> GSEPTFVVNASLLPSKVLGLQVQRPQSFNYQPGDYLFIKCPGISKFEWHPFTISSAPEMPDVLTLHIRAVGSWTGKLYQLI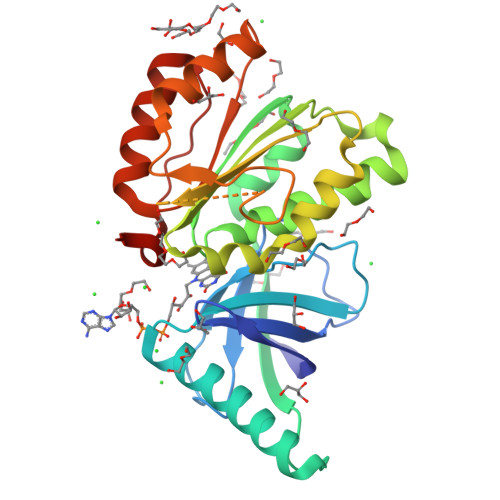REQREEWIRSGSSQSLPGVPVYIDGPYGTPSTHIFESKYAILICAGIGVTPFASILKSILHRNQQNPAKMPLKKVHFYWLNREQKAFEWFVELLSKIEAEDTNNLFDLNLYLTGAQQKSDMKSSTLFVAMDLMHQETKVDLITGLKSRTKTGRPDWEEIFKDVAKQHAPDNVEVFFCGPTGLALQLRHLCTKYGFGYRKENFPWLELAAA>HHHHHHMIIKNYSYARQNLKALMTKVNDDSDMVTVTSTDDKNVVIMSESDYNSMMETLYLQQNPNNAEHLAQSIADLERGKTITKDIDV[4x];>[4x]MARLNITFSPQAFEDYKYFQQNDKKMVKKINELLKSIDRNGALEGIGKPEKLKSNLTGYYSRRINHEHRLV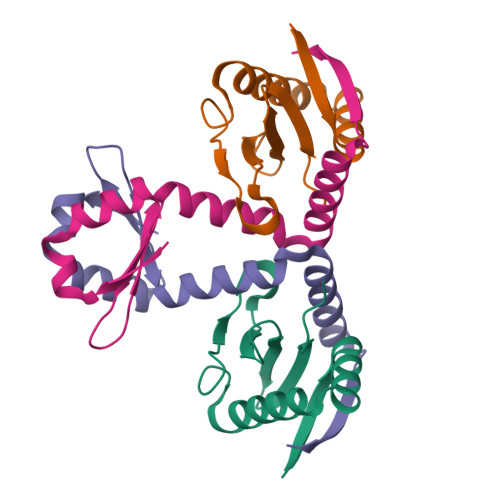YTVDDNHIKIASCKYHY>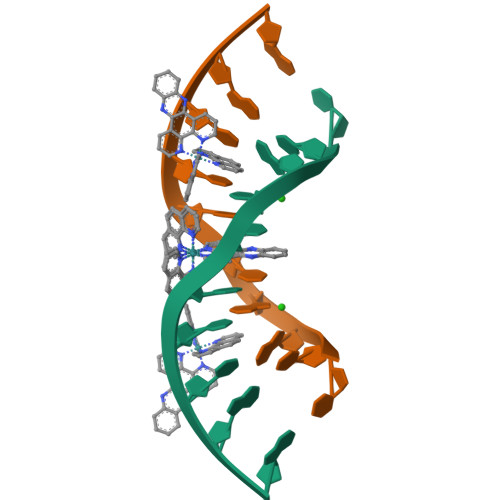 TCGGTACCGA> MSGVPFPSRVIGDLDYSNLLNIGQEEAIRCVLNAYPNIGLEATNLGRARRIVQRALNDNGMDGNKVMLAYTSNLISSGLRDTFACLARENRIGAVVTTAGGVEEDVIKCLGDTLVGDFALNDHALRNNGLNRVGNLLVPNDNYRNFEDFFVPLLRRLHEQQRDSRWTTKTTPSQIIAEIGAALESVRPNDCGSSLIYWCYRNDIPVFSPAFTDGSMGDMIYFYNYSRKGLVVDPVPDVRRLRQLGCKSTNVGRITCI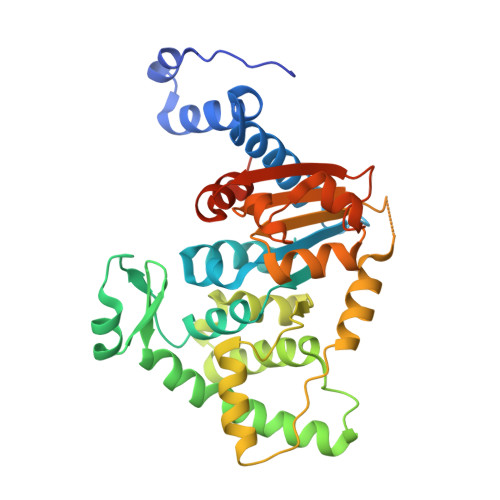VLGAGLPKHHLLRNVQADAVVYVTTGSDADGCESSCNVMADRANGLLSPNCDVVRVHGDATIISPLLLLRSSDGKEKVGVREDGN> MFHFIPSWYNENRTWYDNNYLWYFKPTNVGFDDTINQMKMFDYAGKESRLVVLNYMPNLRYYLHRYDLLESGYYSVFDDIQEIGNVRQQMIDFRQLNWPEGVDFTYTPFIVLVKKSGDLIAKVQFGEEGNLTHIDYFANEQIAKKYLFDDRGFLSSILYYDNGGEAYQDYLAPSGERIMREYLREGDHHVEINPKKAIHFLKLSYSDIEELIREKYLTYLHKEVSKSDTIIVSFNQVHNAFIVGNTSKGNLILSVFSERNNAHNVLEDYSSLSRADAIICDRLDIAAQLKEKIDKPVVHVSPFDTRLALGKSNQVRDLEIYFVVDRLSHKELQKSLTSLYKVMLKNNDIKVTFVSYEREFESRQLTYDYLKEATKVFDQKFFSLSDDDANQVLMQSDEVEKEKTRLSFTHPLSETDIINRLEYVRLIIDISKIPDLYTQIAGISSGIPQINTILTEFVEHRKNGYI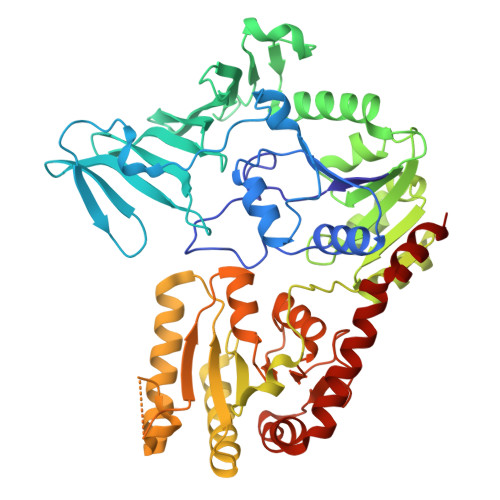IEEIQELEKAIPYYCEQLTNWNRSLIYSIDKINDYTGGQLVERIINSY> AAAVRENALLSSSLWVNVALAGIAILVFVYMGRTIRPGRPRLIWGATLMIPLVSISSYLGLLSGLTVGMIEMPAGHALAGEMVRSQWGRYLTWALSTPMILLALGLLADVDLGSLFTVIAADIGMCVTGLAAAMTTSALLFRWAFYAISCAFFVVVLSALVTDWAASASSAGTAEIFDTLRVLTVVLWLGYP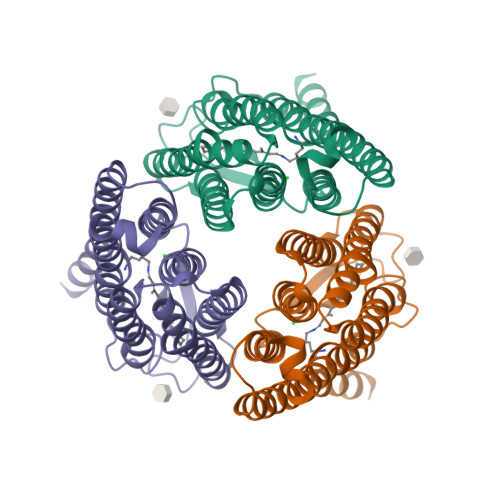IVWAVGVEGLALVQSVGVTSWAYSVLDVFAKYVFAFILLRWVANNERTVAVAGQTLGTMSSDDHHHHHH DHAR catalyses the reduction of DHA to AsA using glutathione (GSH) as a hydrogen donor before the spontaneous hydrolysis of DHA to irreversibly form 2,3-diketogulonic acid. To expand our knowledge of the underlying molecular mechanism of OsDHAR activity against ROS, high-resolution crystal structures of the apo-form, AsA-bound, and GSH-bound OsDHAR were examined at 1.9, 1.7, and 1.7 Å resolution, respectively. The structure shows that the asymmetric unit contains one molecule of OsDHAR and adopted a canonical GST fold, consisting of three β-strands and three α-helices in the N-terminal subdomain (residues 4–84) and six α-helices in the C-terminal subdomain (residues 94–210), although OsDHAR showed modest sequence identity (~20%) with GSTs. Structural comparison studies revealed that Cys20 is a catalytic residue and that Lys8 directly interacts with AsA and GSH to reduce Cys20.

To obtain crystals of the AsA-bound protein, Cys20-mutated OsDHAR (C20S) was used, which lacks reductase activity but exhibits AsA binding activity. The AsA-bound OsDHAR structure was refined at 1.7 Å resolution and contained one molecule of AsA bound to OsDHAR in the asymmetric unit. The AsA bound to a pocket at the cleft that separated the N- and C-domains of OsDHAR. In detail, the 3′-OH and 6′-OH groups on AsA formed hydrogen bonds with the side chain of the Lys8 and Lys210 residues, respectively. In addition, the 5′-OH group of AsA interacted with the OD2 atom of Asp19. The C1′-carbon of the bound AsA was 5.0 Å from Ser20, but rotation of the side chain may produce a suitable distance for catalytic reduction by the Cys20 residue. Structural analyses also revealed that OsDHAR undergoes AsA-associated conformational changes. In particular, the Lys8, Trp207, and Lys210 residues showed structural differences from their corresponding residues compared with the oxidized and GSH-bound structures, and rearrangement of these residues is related to the movements necessary for the interactions involved in AsA binding. In contrast, the bound AsA in OsDHAR is surrounded by α1, α5, and α7, forming the H-site20. The bound AsA in OsDHAR interacts with Lys8 and Lys210 via hydrogen bonds and forms van der Waals interactions with Pro21, Phe104, and Trp207.

> MHHHHHHASENLYFQGAMGVEVCVKAAVGHPDTLGDSPFSQRVLLTLEEKKVPYEMKLIDVQNKPDWFLKISPEGKVPVFNGGDGKWIPDSDVITQVIEEKYPTPSLVTPPEYASVGSKIFSCFTTFLKSKDPNDGSEKALLTELQALEEHLKAHGPFINGQNISAADLSLAPKLYHLQVALEHFKGWKIPEDLTNVHAYTEALFSRESFIKTKAAKEHLIAGWAPKVNA(2~{S})-2-[[(2~{S})-6-[(6-fluoranylpyridin-3-yl)amino]-1-oxidanyl-1,6-bis(oxidanylidene)hexan-2-yl]carbamoylamino]pentanedioic 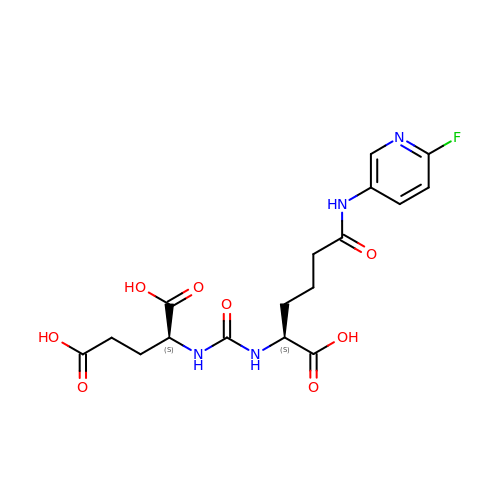acid | C17 H21 F N4 O8 | OAJLMFWIFAWMDP-QWRGUYRKSA-N> MASPAPSWTRLDPQQERDVRELIRLVSGVQDEADPNFQLALHFAWSNFRFHRFLDVNSHKVEKTIEGIYEKFIIHSDLSKAASWKRLTDEFLNASLPSIKEIKTDAHYSILSLLLCLSDSPSNSNYVETPRNKEVEKKDDFDWGKYLMEGEEIDLGPNVDTPNWSEESEDEDDPQPLSREDSGIQVDRTPLEEQDQSRKPASRVSWKVDEPDARSWLEQHVVRQYWTTRSSKFPHSLHLHSNLAAVWDQHLYSSDPL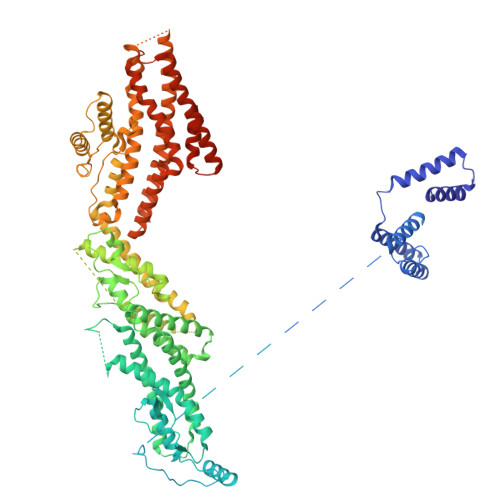YVPDDRVSVTETQVIRETLWLLSGVKKLFIFQLIDGKVAVRNNIMVTHLTHSCLRSVLEQIAAYGQVVFRLQEFIDEVMGHSSESTLPGNGSVPKKSTDAPFRTYQAFMWALYKYFISFKEELSEIEKCIINNDTTVTLAIVVDKLSPRLAQLKVLHKVFSTGVAEVPPDTRNVVRASHLLNTLYKAILEYDNVGEASEQTVSLLFSLWVETVRPYLQIVDEWIVHGHLCDGAREFIIQRNKNVPVNHRDFWYATYTLYSVSEKTENEEKMSDNASASSGSDQGPSSRQHTMVSFLKPVLKQIIMAGKSMQLLKNLQCAESTTCQAMARDAERKSLYTLFLESVQSRLRHGEDATAQALTEQQATRETLIKMQSIAERHLELDDVHDPLLAINFARLYLEQSDFHEKFAGGDICVDRSSESVTCQTFELTLRSCLYPHIDKQYLDCCGNLMRTLKKDYRLVEYLQAMRNFFLMEGGDTMYDFYTSIFDKIREKETWQNVSFLNVQLQEAVGQRYPEDSSRLSISFENTDTAKKKLPVHTLDGLTLSYKVPWPVDIVISLECQKIYNQVFLLLLQIKWAKYSLDVLLFGELASSAEKPQSKEGLLSGQDTAAQFGPQKEPVRQQIHRMFLLRVKLMHFVNSLHNYIMTRILHSTGLEFQHQVEEAKDLDQLIKIHYRYLSTIHDRCLLREKVSFVKEAIMKVLNLALMFADGWQAGLGAWQMESIEKMESDFKNCHMFLVTILNKAVCRGSFPHLESLALSLMAGMEQKREDDLFNHTWGQGDLPNYTCAVRLLGVRKGGGTRPK YceI proteins are a family of bacterial lipocalins (BCNs), which are small proteins widely conserved in Gram-negative and Gram-positive bacteria but whose physiological role is unclear. In this study, we discovered that secreted BCNs contribute to antibiotic resistance by capturing and neutralizing antibiotics in the bacterial milieu. Visual inspection and structural alignments by the DALI server confirmed a barrel-shaped lipocalin fold for both proteins. An octaprenyl pyrophosphate was bound within a long, hydrophobic tunnel extending from one end of the barrel in each structure.

BcnA is a secreted bacterial lipocalin required for full resistance of B. cenocepacia to different classes of antibiotics. To elucidate the mode of binding of antibiotics within BCNs, we first solved the X-ray crystal structures of BcnA and BcnB to 1.4- and 1.6-Å resolutions, respectively. Analysis with the PDBePISA server predicted that BcnA is a monomer, while BcnB is a dimer, by crystallographic symmetry (~2,840 Å2 of buried surface area including a portion of the tunnel opening). Superposition of BcnA chain A and BcnB chain C (148 Cα atoms, 22% sequence identity) resulted in a root mean square deviation (RMSD) of 1.66 Å. The largest structural differences observed were located in two of the loops that make up the tunnel opening. Using the established crystallographic structures, we applied molecular modeling and docking calculations to predict BCN binding modes of antibiotics. These studies suggested two distinct docked binding modes for BcnA. One binding mode involved residues in the rim of the lipocalin pocket. The second binding mode was predicted for more lipophilic molecules (e.g., Nile red), occurring deeper inside the lipophilic tunnel. Docking of α-tocopherol showed its alkyl chain buried in the BcnA tunnel and its cyclic head placed toward the entrance, similar to the Nile red binding pose.

>HMDVDLAKSKVSAVSKQMNVPTEGAFKKFSAQVKFDPAKAAQGSAQMTIDVASFDLGDKMYNDQVAGKDWFDAKTYPQATFVSSAIAPAGGNKYNVTGKLTIKGKAETVTVPVTVAQNGATQTFDGVLPIKRSAFNVGTGEWKDTSIVADEVQIKFHLVAT[2x]During energy production in Desulfitobacterium hafniense, MtgA catalyzes the methyl transfer from methylcobalamin (Cbl‐CH3) to THF in the catabolism of glycine betaine (GB). Despite its lack of sequence identity with known structures, we could show that MtgA forms a homodimeric complex of two TIM barrels. The topology of each subunit is characterized by a funnel of eight parallel β‐sheets connected by α‐helices on the outside that form a complex of two perpendicularly oriented TIM barrels. The active‐site cavity is located inside the hydrophilic core of each barrel.

5 of THF and activates it for attack of the incoming Cbl‐bound CH3 group. These first mechanistic insights were confirmed by replacing Asp102 with alanine. In the MtgA D102A mutant, methyl transfer from Cbl‐CH3 to THF is abolished as compared to the wild‐type (WT) enzyme. X‐ray structure analysis of mutant MtgA in complex with THF‐CH3 gave further insights into the reaction trajectory. Therefore, both mutants mimic product formation at a late reaction state.

>[2x]GSFKFTAQQHVYDINGVKVGGQPGEYPTVLIGSIFYRGHKIVSDGQKGIFDKDAAKALLDQEAELSAETGNPFIIDVLGESVEALTKYVEFILENTTAPFLLASISPDVRVGALKNLGKDPEIQKRLIYNSIEEHYTEEELAAIKEAGLKTAVILAFSKKALKPNARIDLLQGKDDKEGLIAAAKRAGIEQFLVDPGVLDVASNSWTTEAINVVKEQFGYPGGCAPSNAVYLWKKMRSKGTPFFEVAGAAVFTYPITQGADFILYGPMMNAPWVYRAIATTDAMIAYNNKLTGVKMGTTEHPLLKIF> GHHHHHHGSGSGENLYFQGGGSGVSLGQALLILSVAALLGTTVEEAVKRALWLKTKLGVSLEQAARTLSVAAYLGTTVEEAVKRALKLKTKLGVSLEQALLILFAAAALGTTVEEAVKRALKLKTKLGVSLEQALLILWTAVELGTTVEEAVKRALKLKTKLGVSLGQAQAILVVAAELGTTVEEAVYRALKLKTKLGVSLGQALLILEVAAKLGTTVEEAVKRALKLTTKLG

Here we address these limitations by introducing an artificial metathase—an artificial metalloenzyme designed for ring-closing metathesis—for whole-cell biocatalysis. Our approach integrates a tailored metal cofactor into a hyper-stable, de novo-designed protein. By combining computational design with genetic optimization, a binding affinity (KD ≤ 0.2 μM) between the protein scaffold and cofactor is achieved through supramolecular anchoring. From the catalyst perspective, we sought to address this challenge by designing a derivative of the Hoveyda–Grubbs catalyst (hereafter Ru1) that contains a polar motif, aimed at interacting via H-bonds with the protein, as well as improving the cofactor solubility in aqueous media.

For the fifth round, we screened a fragment shuffling library (540 colonies) by randomly recombining the beneficial mutations from third and fourth rounds. This led to the identification of variant Ru1·R5 (that is, Ru1·dnTRP_18_E4G/F43R/I44T/F116W/A119V/E144G/E179G/K206T) that afforded TON = 339 ± 34 and 570 ± 25 in CFE and purified form, respectively. The evolved metathase Ru1·R5 maintained nearly half of its activity at pH 6.0 (versus pH 4.2), whereas Ru1·R0 lost nearly ninety percent of its activity. The highest TON was achieved at 50 °C. At pH 3.6 and 50 °C, Ru1·R5-ΔHis afforded a TON of 1,028 ± 159. The X-ray structure of Ru1·R5-ΔHis displays close structural similarity to Ru1·R0-ΔHis, with a backbone ΔHis of 0.6 Å and a Ru atom deviation of 1.0 Å between the two structures. Notably, compared with Ru1·R0-ΔHis, the evolved variant Ru1·R5-ΔHis features an expanded and less hydrophilic channel leading to the active site, which results from the three critical E4G, E144G and E179G mutations. These probably contribute to the increased affinity of dnTRP_R5-ΔHis (versus dnTRP_R0-ΔHis) and hinder the approach of hydrophilic species (including GSH, OH− and so on) that lead to cofactor inhibition. In developing a computational model of Ru1·R5-ΔHis, the structure was predicted using AlphaFold2 and further refined using Rosetta FastRelax in the presence of Ru1. Yet, the resulting models did not accurately reflect the deeper placement of the Ru1 cofactor as observed in the crystal structure. In contrast to the free cofactor Ru1, the dnTRP-ΔHis host protein protects the thiophilic Ru1 cofactor from poisoning by GSH: at [GSH] = 1.28 mM, Ru1·R5-ΔHis maintains > 20% of its RCM activity, whereas Ru1 is completely inactivated at [GSH] ≥ 40 μM. Guided by the X-ray structure of Ru1·R5-ΔHis, we selected four residues (L8, L113, A148 and L183) located in the proximity of the ruthenium for randomization with 17 amino acid residues (except Cys and Pro).> MAKPTQDSQEKVSIEQQLAVESIRKFLNSKTSYDVLPVSYRLIVLDTSLLVKKSLNVLLQNSIVSAPLWDSKTSRFAGLLTTTDFINVIQYYFSNPDKFELVDKLQLDGLKDIERALGVDQLDTASIHPSRPLFEACLKMLESRSGRIPLIDQDE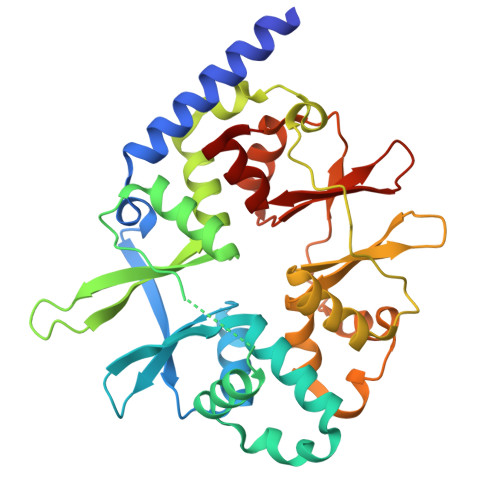ETHREIVVSVLTQYRILKFVALNCRETHFLKIPIGDLNIITQDNMKSCQMTTPVIDVIQMLTQGRVSSVPIIDENGYLINVYEAYDVLGLIKGGIYNDLSLSVGEALMRRSDDFEGVYTCTKNDKLSTIMDNIRKARVHRFFVVDDVGRLVGVLTLSDILKYILLGSN>[5x]GMLLSTDIWVAALIRRA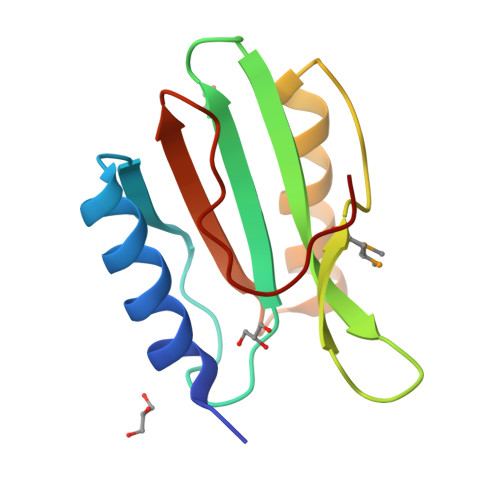ELGGAFATVARKGDARAGAVLVKAVDRREGTARLFSEATRGDGERFWMQPVRSTFEPDLDAYAERAARIDPDIWVVEIEDRDGRHFLTEPVES>VDLSNLPRVKHTLVPPPFAHAHEQVAASGPVINEFEMRIIEKEVQLDEDAYLQAMTFDGSIPGPLMIVHEGDYVELTLINPPENTMPHNIDFHAATGALGGGGLTLINPGEKVVLRFKATRAGAFVYHCAPGGPMIPWHVVSGTAGCIMVLPRDGLKDHEGKPVRYDTVYYIGESDHYIPKDEDGTYMRFSDPSEGYEDMVAVMDTLIPSHIVFNGAVGALTGEGALKAKVGDNVLFVHSQPNRDSRPHLIGGHGDLVWETGKFHNAPERDLETW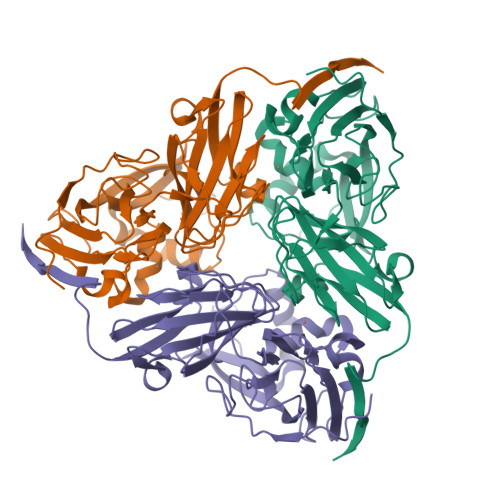FIRGGTAGAALYKFLQPGVYAYVNHNLIEAVHKGATAHVLVEGEWDNDLMEQVVAPVGL[3x]> MSTNKVNKERTFLAVKPDGVARGLVGEIIARYEKKGFVLVGLK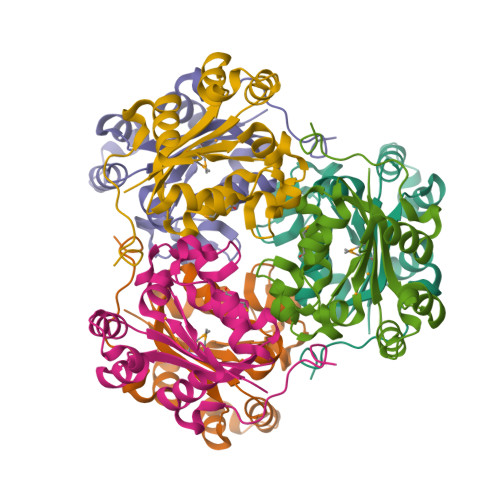QLVPTKDLAESHYAEHKERPFFGGLVSFITSGPVVAMVFEGKGVVASARLMIGVTNPLASAPGSIRGDFGVDVGRNIIUGSDSVESANREIALWFKPEELLTEVKPNPNLYE> GRSLHHKSALFSCVTDPKEMHCHENWSLSPEEFEIWDRLYRLKENDGVKEPILPHTRFETLENLDKTSKPEEEAAHKLSLSEWSIWQSRPFPTSMVDHSDRCYHFISVMELIEVMRQE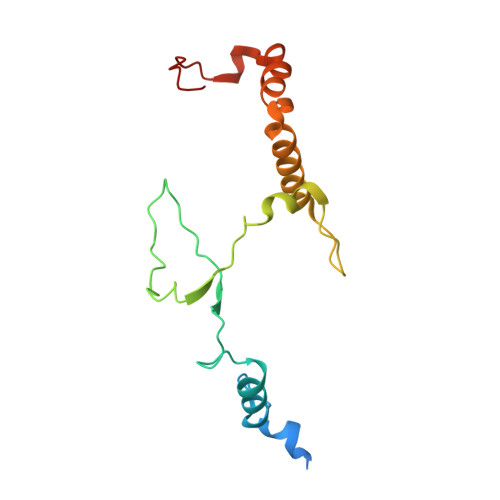QGDCSYELELQPHLRIEDIHVRRNKGHLSP(2-{[2-(2,6-dimethylphenoxy)ethyl]sulfanyl}-1H-benzimidazol-1-yl)acetic 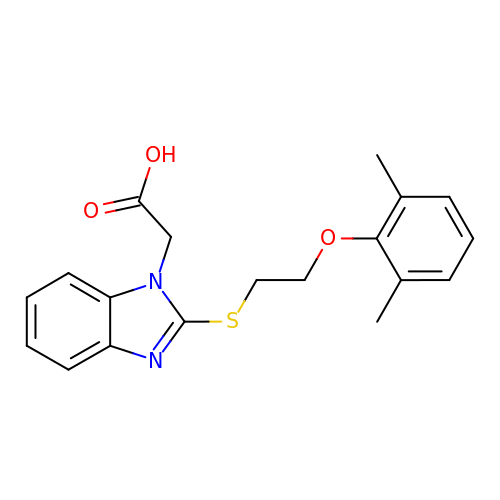acid | C19 H20 N2 O3 S | ZAHFRMHMWCBLOL-UHFFFAOYSA-N7-methyl-3-methylidene-oct-1-ene 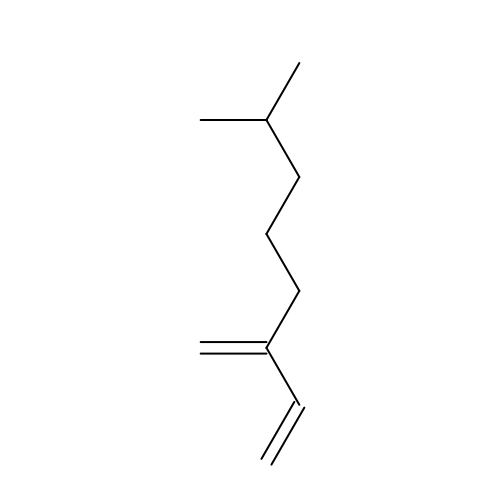| C10 H18 | CIGQIEANONTNMS-UHFFFAOYSA-N> RDEEDLQRYIDVTRGEIFFSRGVILVEGDAERFIVPAFAEVLNIP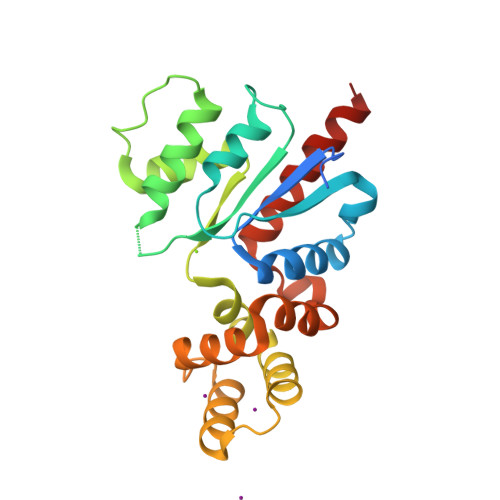LDMLGITVCSVGGTNFTPYVKLLGPEGLNIPHVILTDRDPTNGNHPLVRRRLINVLDVIEGGVDHEELDADEVIKLAEQYGYFVNENTLEPELFAGGLAEDMQEVIREELPRLRRETLNALQQWVDDPAQIDEDLLLRLIERIGKGRFAQALAPSVSEDVCPAYIRSALEHIRDAIALEHHHHHH> NIQTQLDNLRKTLRQYEYEYHVLDNPSVPDSEYDRLFHQLKALELEHPEFLTSDSPTQRVGAKPLSGFSQIRHEIPMLSLDNAFSDAEFNAFVARIEDRLILLPAPLTFCCEPKLDGLAVSILYVNGELTQAATRGDGTTGEDITANIRTIRNVPLQLLTDNPPARLEVRGEVFMPHAGFERLNKYALEHNEKTFANPRNAAAGSLRQLDPNITSKR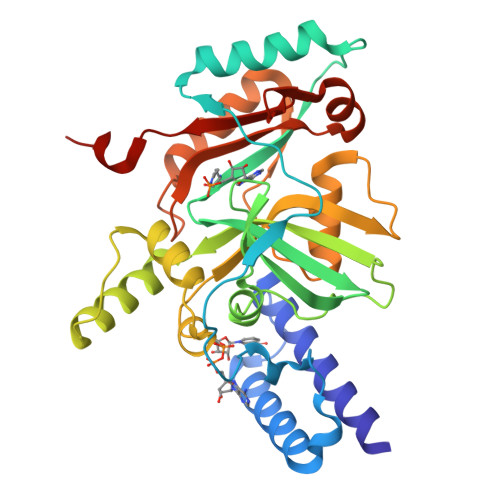PLVLNAYGIGIAEGVDLPTTHYARLQWLKSIGIPVNPEIRLCNGADEVLGFYRDIQNKRSSLGYDIDGTVLKINDIALQNELGFISKAPRWAIAYKFPAQEELTL>KNLNPKKFSIHDQDHKVLVLDSGNLIAVPDKNYIRPEIFFALASSLSSASAEKGSPILLGVSKGEFCLYCDKDKGQSHPSLQLKKEKLMKLAAQKESARRPFIFYRAQVGSWNMLESAAHPGWFICTSCNCNEPVGVTDKFEN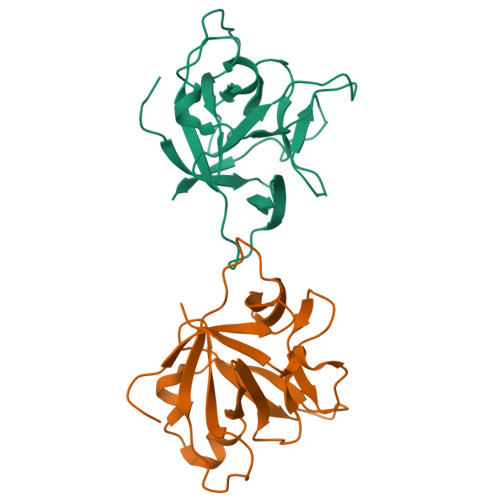RKHIEFSFQPV[2x]Nucleophosmin 1 (NPM1) is an abundant nucleolar protein that forms large oligomers and undergoes liquid–liquid phase separation by binding RNA or ribosomal proteins. It provides the scaffold for ribosome assembly but also prevents protein aggregation as part of the cellular stress response. NPM1 has a modular structure with folded N-terminal and C-terminal domains (NTD, residues 1 to 120, and CTD, residues 240 to 294) linked by an intrinsically disordered region (IDR, residues 120 to 240). The N-terminal domain adopts a β-sheet sandwich fold and assembles into pentamers that can form end-to-end decamers.

To better understand how the CTD associates with other parts of NPM1, we turned to cryo-electron microscopy (cryo-EM). Using physiological conditions (pH 7.5 and 150 mM NaCl), we obtained electron density maps that allowed a reconstruction of the NTD with a resolution of 2.6 Å. Comparison to the crystal structure revealed a virtually identical fold, including sidechain orientations, except for the loop covering residues 34 to 39, which makes up the A1 tract. In the X-ray structure, it is stabilized via crystal contacts with the neighboring pentamer. In the cryo-EM density maps, the loop is too flexible for a confident reconstruction, suggesting that not only the A2 and A3 tracts but even the A1 tract in the NTD is disordered. Free CTDs attached to the disordered linker are too small (less than 9 kDa) to be resolved on their own. Interestingly, we obtained two distinct 3D classes, one with an additional density above the acidic side of the pentamer, off-center from central cavity. Strikingly, nearly all particles in this class had another NTD pentamer in the proximity. The extra density is connected to the pentamer via the A2 tract of a single NTD and can therefore not be attributed to the disordered regions of each protomer. Placement of the top-scoring complex between the CTD and the A2 tract into the EM map showed a good agreement between the unassigned density, the helical acidic region of the IDR, and the approximate location of the CTD.

>SMEDSMDMDMSPLRPQNYLFGCELKADKDYHFKVDNDENEHQLSLRTVSLGAGAKDELHIVEAEAMNYEGSPIKVTLATLKMSVQPTVSLGGFEITPPVVLRLKCGSGPVHISGQHLVAVEEDAESEDEEEEDVKLLSISGKRSAPGGGSKVPQKKVKLAADEDDDDDDEEDDDEDDDDDDFDDEEAEEKAPVKKSIRDTPAKNAQKSNQNGKDSKPSSTPRSKGQESFKKQEKTPKTPKGPSSVEDIKAKMQASIEKGGSLPKVEAKFINYVKNCFRMTDQEAIQDLWQWRKSL[5x]> MADETIAIVDADATAETRSLLSYLDGVRGEGILFGHQHTTSFGLTTGPTDGTTSDVKNVTGDFPAVFGWDTLIIEGNERPGLAENTRDENIALFADYIRKADAIGGVNTVSAHVENFVTGGSFYDTSGDTLRAVLPGGSHHAELVAYLDDIAELADASRRDDGTLIPIVFRPWHENAGSWFWWGAAYGSPGEYQELYRFTVEYLRDVKGVSNFLYAWGPGGGFGGNRDV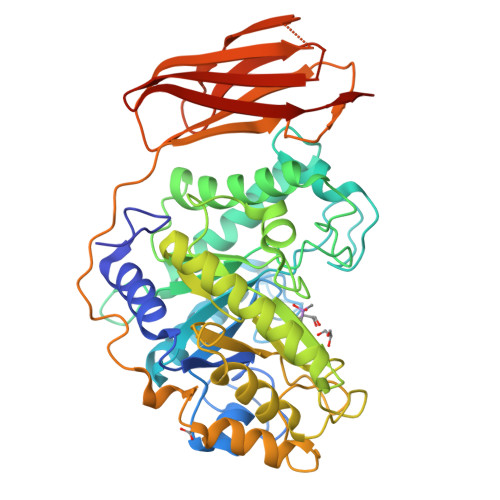YLRTYPGDAFVDVLGLDTYDSTGSDAFLAGLVADLRMIAEIADEKGKVSAFTEFGVSGGVGTNGSSPAQWFTKVLAAIKADPVASRNAYMETWANFDAGQHFVPVPGDALLEDFQAYAADPFTLFASEVTGAFDRTVAAAPAQPVVHIASPADGARVASAPTTVRVRVGGTDVQSVTVEVAQGGTVVDTLDLAYDGALWWTAPWSPTSAQLDNSTYTVTATATTAAGTLDVTNEVAAALEHHHHHH>[8x]GT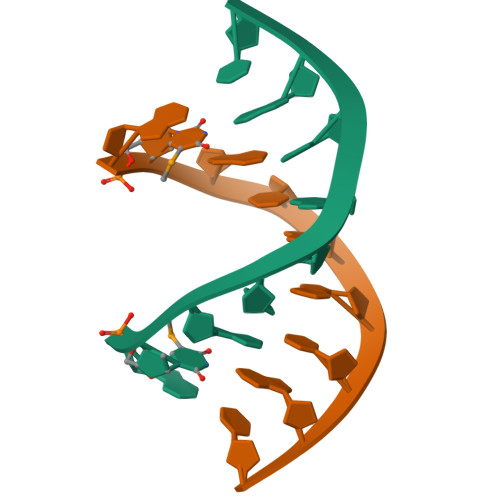GTXACAC>[2x]MKKGHHHHHHLVPRGSRKKIFKPEELRQALMPTLEALYRQDPESLPFRQPVDPQLLGIPDYFDIVKNPMDLSTIKRKLDTGQYQEPWQYVDDVWLMFNNAWLYNRKTSRVYKF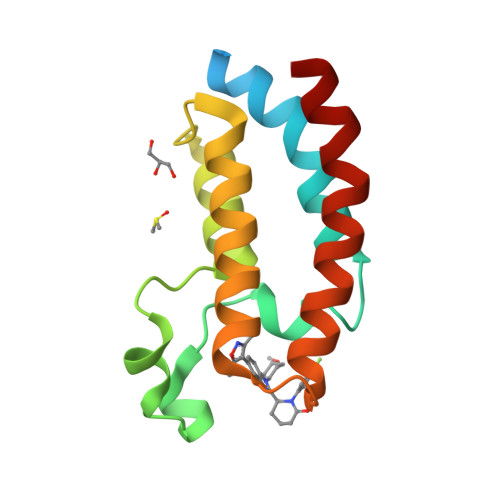CSKLAEVFEQEIDPVMQSLG>NEFSASFKGTDIQEFINIVGRNLEKTIIVDPSVRGKVDVRSFDTLNEEQYYSFFLSVLEVYGFAVVEMDNGVLKVIKSKDAKTSAIPVLSGEERANGDEVITQVVAVKNVSVRELSPLLRQLIDNAGAGNVVHYDPANIILITGRAAVVNRLAEIIRRVDQAGDKEIEVVELNNASAAEMVRIVEALNKTTDAQNTPEFLKPKFVADERTNSILISGDPKVRERLKRLIKQLDVEMAAKGNNRVVYLKYAKAEDLVEVLKGVSENLQAEKGTGQPTTSKRNEVMIAAHADTNSLVLTAPQDIMNAMLEVIGQLDIRRAQVLIEALIVEMAEGDGI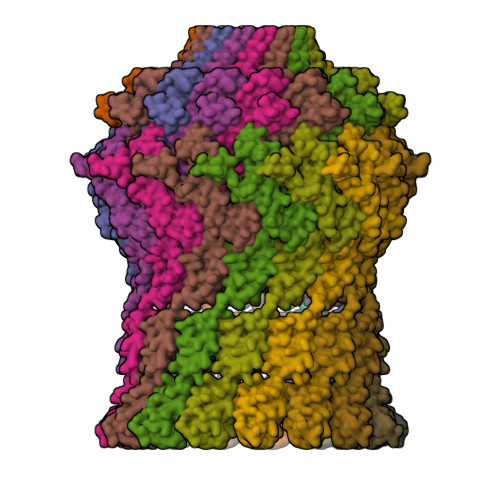NLGVQWGSLESGSVIQYGNTGASIGNVMIGLEEAKDTTQTKAVYDTNNNFLRNETTTTKGDYTKLASALSSIQGAAVSIAMGDWTALINAVSNDSSSNILSSPSITVMDNGEASFIVGEEVPVITGSTAGSNNDNPFQTVDRKEVGIKLKVVPQINEGNSVQLNIEQEVSNVLGANGAVDVRFAKRQLNTSVMVQDGQMLVLGGLIDERALESESKVPLLGDIPLLGQLFRSTSSQVEKKNLMVFIKPTIIRDGVTADGITQRKYNYIRAEQLFRAEKGLRLLDDASVPVLPKFGDDRRHSPEIQAFIEQMEAKQ[15x]> PRRGAVAHANSIVQQLVSEGADISHTRNMLRNAMNGDAVAFSRVEQNIFRQHFPNMPMHGISRDSELAIELRGALRRAVHQQ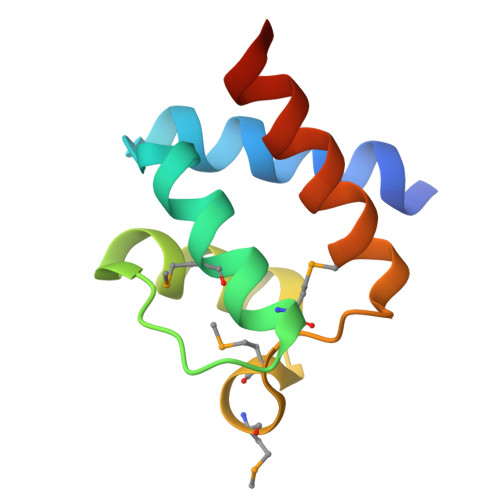AAS>[4x]GATDSATAAPAAAATTQVQKEAADVLQVAVQGANAMRDIQFARLALFHGQPDSAKKLTDDAAALLAADDASWAKFVKTDAKAKMIADRYVIINASIALSEDYVATPEKESAIQSANEKLAK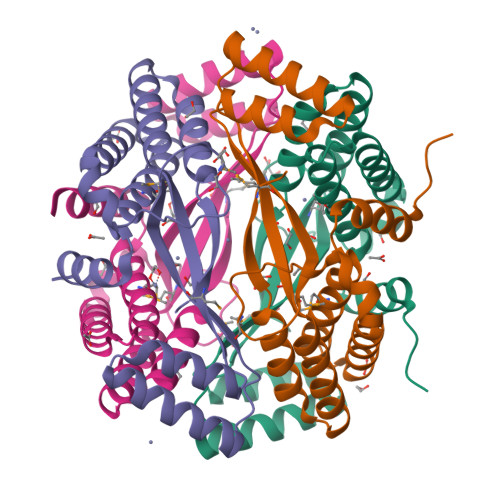GDQKGAIDTLRLAGIGVIENQYLMPLNQTRKAVAQSQELLKAGKYYEANLVLKGAEEGIVVDSEMLVAGN>[2x]MAKSDVFHLGLTKNDLQGATLAIVPGDPQRVEKIAKLMDNPVHLASHREFTSWRAELDGKAVIVCSTGIGGPSTSIAVEELAQLGVRTFLRIGTTGAIQPHINVGDVLVTTAAVRLDGASLHFAPMEFPAVADFSC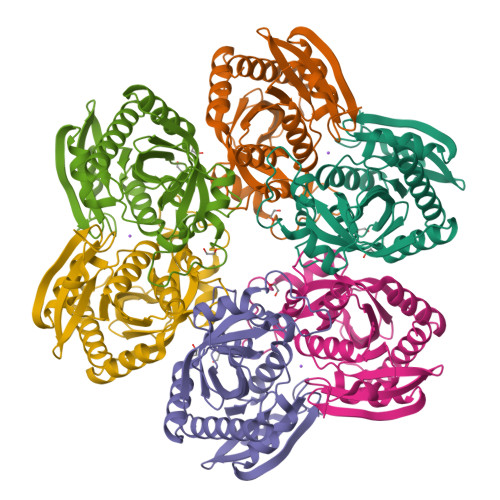TTALVNAAKSVGATTHIGITASSDTFYPGQERYDTFSGRVVRHFKGSMEEWQSMGVMNYEMESATLLTMCASQGLRAGMVAGVIVNRTQQEIPNEETMKATESHAVKIVVEAARHLL>[3x]GPMNKYTIAIDLGYGQIKGINQDNKRVIFPSIISSGKDRSLDTDFNSDDNIVDNIHVKILDEYFNEKEYFVGELAKRQPSNSSFIN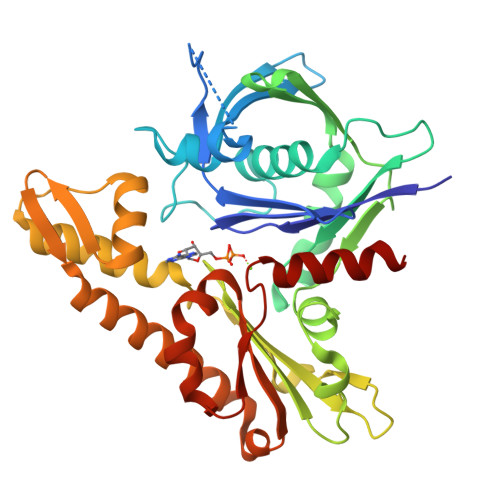RDNKINSEENKVLLATALGLLIPNDLPNDTKIHIVTGLPLEHFIKQKQALNDMLKDFEHTIKFVDHNFSRNIKFEESNITLFPQGAGAIFSKINNDISSLLIKETFIGLIDVGFKTTDIVVFRINKDKEPVFEQEMSATLDGLGMINIYNTMDKAFTDNSRDGSKLNTEQLMLLCEEGKIFFKGDYIDLKKDLIKARKTLSTNIINKADGLWGDDKNSFNSIMIAGGGGKVLYNHLKLIEPNMCQLIDNPEFANAIGYLEFGKQFK>MTHQTHTIAESNNFIVLDKYIKAEPTGDSYQSESDLERELIQDLRNQGYEFISVKSQSAMLANVREQLQNLNGVVFNDSEWRRFTEQYLD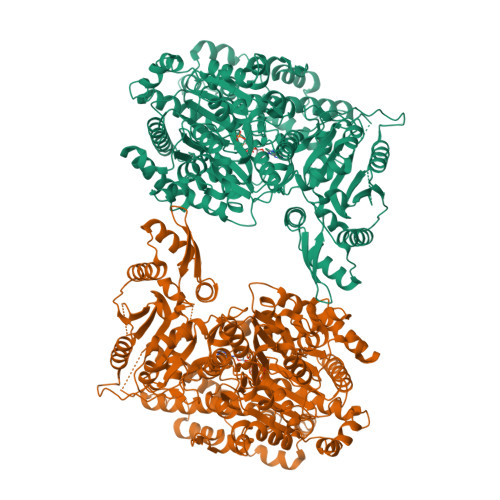NPSDGILDKTRKIHIDYICDFIFDDERLENIYLIDKKNLMRNKVQIIQQFEQAGSHANRYDVTILVNGLPLVQIHLKKRGVAIREAFNQIHRYSKESFNSENSLFKYLQLFVISNGTDTRYFANTTKRDKNSFDFTMNWAKSDNTLIKDLKDFTATCFQKHTLLNVLVNYSVFDSSQTLLVMRPYQIAATERILWKIKSSFTAKNWSKPESGGYIWHTTGSGKTLTSFKAARLATELDFIDKVFFVVDRKDLDYQTMKEYQRFSPDSVNGSENTAGLKRNLDKDDNKIIVTTIQKLNNLMKAESDLPVYNQQVVFIFDECHRSQFGEAQKNLKKKFKRYYQFGFTGTPIFPENALGSETTASVFGRELHSYVITDAIRDEKVLKFKVDYNDVRPQFKSLETETDEKKLSAAENQQAFLHPMRIQEITQYILNNFRQKTHRTFPGSKGFNAMLAVSSVDAAKAYYATFKRLQEEAANKSATYKPLRIATIFSFAANEEQNAIGEISDETFDTSAMDSSAKEFLDAAIREYNSHFKTNFSTDSNGFQNYYRDLAQRVKNQDIDLLIVVGMFLTGFDAPTLNTLFVDKNLRYHGLMQAFSRTNRIYDATKTFGNIVTFRDLERSTIDAITLFGDKNTKNVVLEKSYTEYMEGFTDAATGEAKRGFMTVVSELEQRFPDPTSIESEKEKKDFVKLFGEYLRAENILQNYDEFATLKALQQIDLSDPVAVEKFKAEHYVDDEKFAELQTIRLPADRKIQDYRSAYNDIRDWQRREKEAEKKEKSTTDWDDVVFEVDLLKSQEINLDYILGLIFEHNRQNKGKGEMIEEVKRLIRSSLGNRAKEGLVVDFIQQTNLDDLPDKASIIDAFFTFAQREQQREAEALIKEENLNEDAAKRYIRTSLKREYATENGTELNETLPKLSPLNPQYKTKKQAVFQKIVSFIEKFKGVGGKI[2x]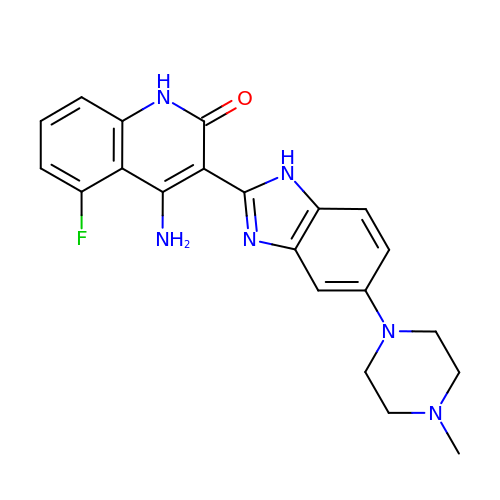4-amino-5-fluoro-3-[5-(4-methylpiperazin-1-yl)-1H-benzimidazol-2-yl]quinolin-2(1H)-one | C21 H21 F N6 O | PIQCTGMSNWUMAF-UHFFFAOYSA-N>MITIDGSYGEGGGQILRTSVALSTITGEPVRIVNIRANRPNPGLRPQHLHAILALKHLANAEVKGAHVGSRELVFIPKKLEAKEISIDIGTAGSITLVLQALLPAMVFAREKVKFRITGGTDVSWSPPVDYLSNVTLFALEKIGIHGEIRVIRRGHYPKGGGIVEGYVEPWNEKRELVAKEYSRIIKIEGISHATNLPSHVAERQARAAKDELLQLKVPIEIRTEISRSIGPGSGIVVWAETDCLRLGGDALGKKGKPAEIVGKEAAQELLDQLKPGHCVDKFLGDQLIPFLAFSGGVIWVSEITNHLKTNIWVVESFLGRIFDVDGNVGEPGKIRVIRR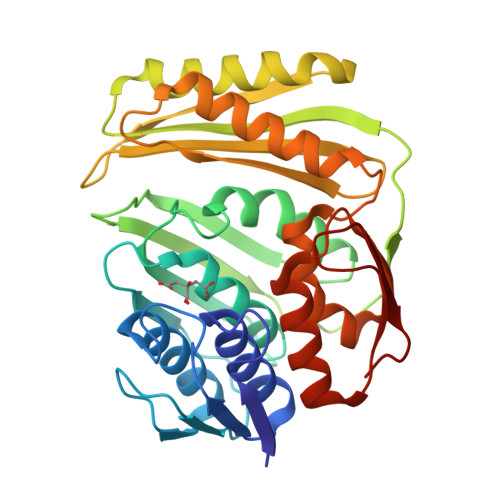V[2x]>[6x]APPCSRCFARAIESSRDLLHRIKDEVGAPGIVVGVSVDGKEVWSEGLGYADVENRVPCKPETVMRIASISKSLTMVALAKLWEAGKLDLDIPVQHYVPEFPEKEYEGEKVSVTTRLLISHLSGIRHYEKDIKKVKEEKAYKALKMMKENVAFEQEKEGKSNEKNDFTKFKTEQENEAKCRNSKPGKKKNDFEQGELYLREKFENS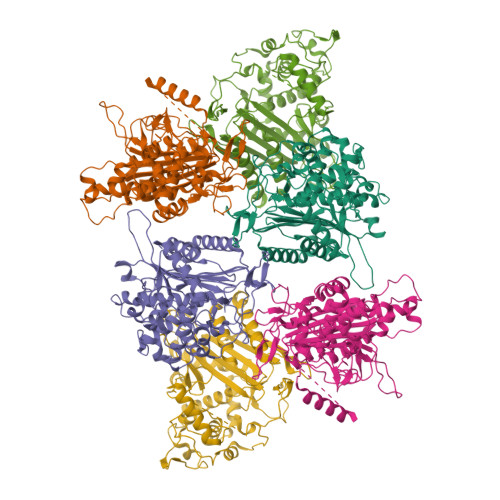IESLRLFKNDPLFFKPGSQFLYSTFGYTLLAAIVERASGCKYLDYMQKIFHDLDMLTTVQEENEPVIYNRARFYVYNKKKRLVNTPYVDNSYKWAGGGFLSTVGDLLKFGNAMLYGYQVGLFKNSNENLLPGYLKPETMVMMWTPVPNTEMSWDKEGKYAMAWGVVERKQTYGSCRKQRHYASHTGGAVGASSVLLVLPEELDTETINNKVPPRGIIVSIICNMQSVGLNSTALKIALEFDKDRSD> MFLGIRDIRAAAGRFALIASVVGLITLLIVMLTGLTQGLGKQNTSAIEALAPHSVVFTTAGGSSPEFTSSEISEQQAERWKDSTPLGVSQTRIESDQNANTTAVMGLPEGTPLPDSVGGFIEQGALLPAELADFLHVRAGDHITLGGATVTVAGTVKTENYSHTPVVWVDTATWQLVSHTKAVGTVLLLNQEPTIQPQDNEVVTDLKGAFQAMPAYKSERSSLLSM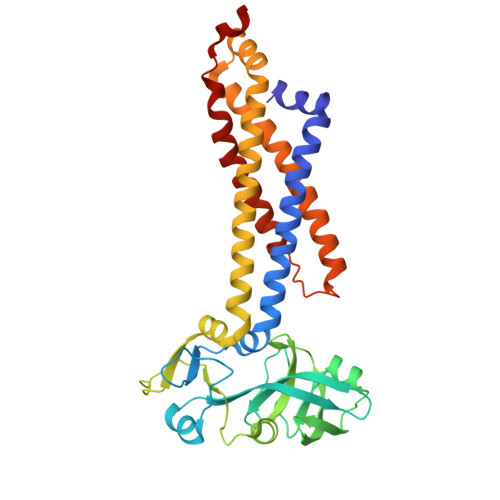QAFLYIISALVTVAFLTVWTLQRTRDIAVLAALGASKRYLLIDALGQAAIILAAGVALGAGIGALLGWLIAGSVPFSLGWVSVLGPALGIWLLGLIGATIAVRNVTKVDPQIALGATA4-{[4-({4-[(E)-2-cyanoethenyl]-2,6-dimethylphenyl}amino)pyrimidin-2-yl]amino}benzonitrile 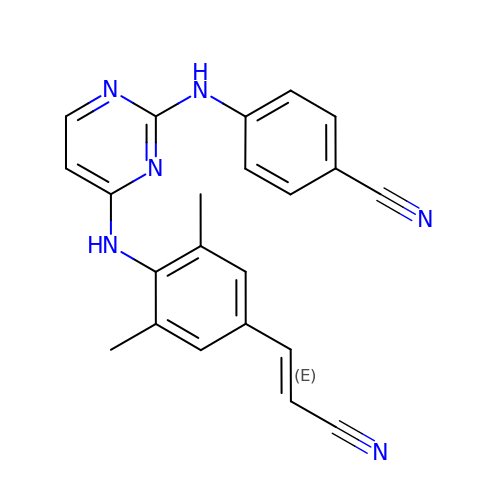| C22 H18 N6 | YIBOMRUWOWDFLG-ONEGZZNKSA-N>SMSFEGKIALVTGASRGIGRAIAETLVARGAKVIGTATSESGAQAISDYLGANGKGLMLNVTDPASIESVLENVRAEFGEVDILVNNAGITRDNLLMRMKDDEWNDIIETNLSSVFRLSKAVMRAMMKKRHGRIITIGSVVGTMGNAGQANYAAAKAGLIGFSKSLAREVASRGITVNVVAPGFIETDMTRALTDEQRAGT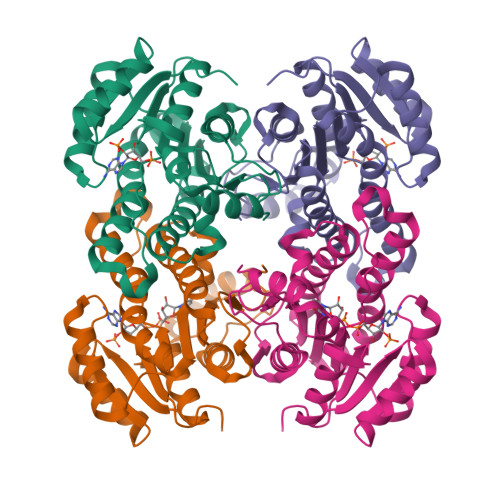LAAVPAGRLGTPNEIASAVAFLASDEASYITGETLHVNGGMYMV[2x]>ESYLSPAQSVKPKINTEEKLPREKLNPPTPSIYLESKRDAFSPVLLQFCTDPRNPITVIRGLAGSLRLNLGLFSTKTLVEASGEHTVEVRTQVQQPSDENWDLTGTRQIWPCESSRSHTTIAKYAQYQASSFQESLQEELEVLFQGPTKAARKSAPATGGGSSGSHHIIKFGTNIDLSDAKRWKPQLQELLKLPAFMRVTSTGNMLSHVGHTILGMNTVQLYMKVPGSRTPGHQENNNFCSVNINIGPGDCEWFAVHEHYWETISAFCDRHGVDYLTGSWWPILDDLYASNIPVYRFVQRPGDLVWINAGTVHWVQATGWCNNIAWNVGPLTAYQYQLALERYEWNEVKNVKSIVPMIHVSWNVARTVKISDPDLFKMIKFCLLQSMKHCQVQRESLVRAGKKIAYQGRVKDEPAYYCNECDVEVFNILFVTSENGSRNTYLVHCEGCARRRSAGLQGVVVLEQY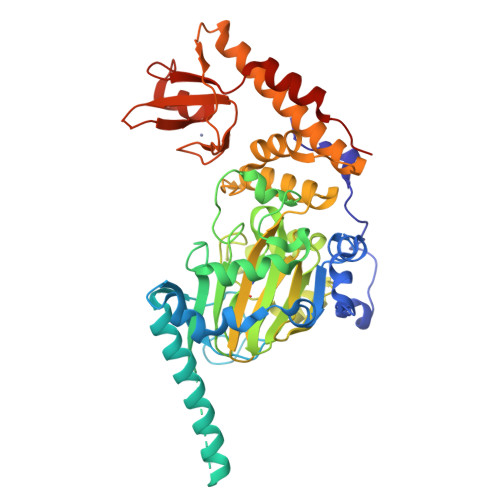RTEELAQAYDAFTLAPASTSR[2x]> GSTPVSEKQLAEVVANTITPLMKAQSVPGMAVAVIYQGKPHYYTFGKADIAANKPVTPQTLFELGSISKTFTGVLGGDAIARGEISLDDAVTRYWPQLTGKQWQGIRMLDLATYTAGGLPLQVPDEVTDNASLLRFYQNWQPQWKPGTTRLYANASIGLFGALAVKPSGMPYEQAMTTRVLKPLKLDHTWINVPKAEEAHYAWGYRDGKAVRVSPGMLDAQAYGVKTNVQDMANWVMANMAPENVADASLKQGIALAQSRYW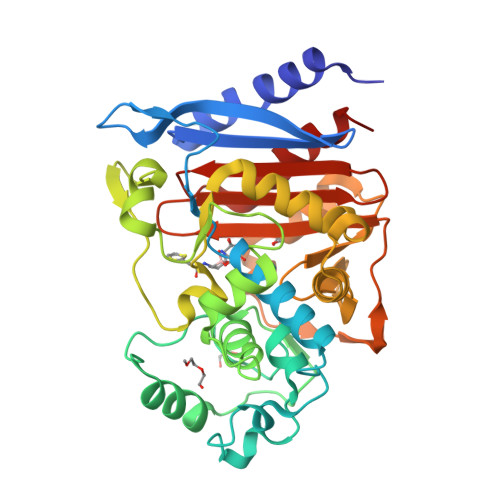RIGSMYQGLGWEMLNWPVEANTVVEGSDSKVALAPLPVAEVNPPAPPVKASWVHKTGSTGGFGSYVAFIPEKQIGIVMLANTSYPNPARVEAAYHILEALQ> GPIPTAPRENSLMFLSTTPDDTVPAYGNVRTPPVNYLPGEITDLLQLARIPTLMAFGRVDAYVPYVAVPTQFDDKPLISFPITLSDPVYQNTLVGAISSNFANYRGCIQITLTFCGPMMARGKFLLSYSPPNGTQPQTLSEAMQCTYSIWDIGLNSSWTFVIPYISPSDYRETR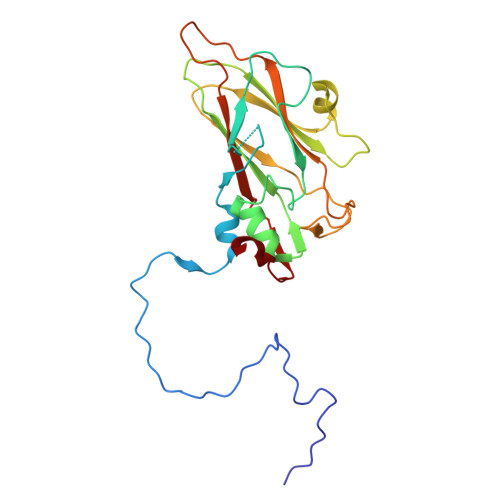AITNSVYSADGWFSLHKLTKITLPPDCPQSPCILFFASAGEDYTLRLPVDCNPSYVF>LRRRYTMASGPQVDNTGGEPAWDSPLRRVLAELNRIPSSRRRAARLFEWLIAPMPPDHFYRRLWEREAVLVRRQDHTYYQGLFSTADLDSMLRNEEVQFGQHLDAARYINGRRETLNPPGRALPAAAWSLYQAGCSLRLLCPQAFSTTVWQFLAVLQEQFGSMAGSNVYLTPPNSQGFAPHYDDIEAFVLQLEGRKLWRVYRPRAPTEELALTSSPNFSQDDLGEPVLQTVLEPGDLLYFPRGFIHQAECQDGVHSLHLTLSTYQRNTWGDFLEAILPLAVQAAMEENVEFRRGLPRDFMDYMGAQHSDSKDPRRTAFMEKVRVLVARLGHFAPVDAVADQRAKDFIHDSLPPVLTDRERALSV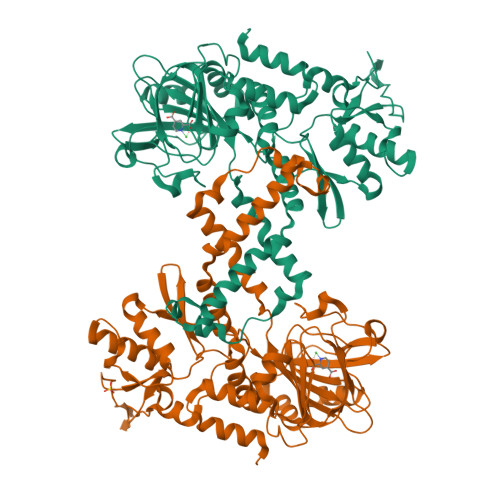YGLPIRWEAGEPVNVGAQLTTETEVHMLQDGIARLVGEGGHLFLYYTVENSRVYHLEEPKCLEIYPQQADAMELLLGSYPEFVRVGDLPCDSVEDQLSLATTLYDKGLLLTKMPLALNAENLYFQ[2x]> SNASSPSSPADWAKKLTDAVLRQKAGETLTAADRDFSNADFRNITFSKILPPSFMERDGDIIKGFNFSNSKFTYSDISHLHFDECRFTYSTLSDVVCSNTKFSNSDMNEVFLQYSITTQQQPSFIDTTLKNTLIRHKANLSGVILNEPDNSSPPSVSGGGNFIRLGDIWLQMPLLWTENAVDGFLNHEHNNGKSILMTIDSLPDKYSQEKVQAMEDLVKSLRGGRLTEACIRPVESSLVSVLAHPPYTQSALISEWLGPVQERFFAHQCQTYNDVPLPAPDTYYQQRILPVLLDSFDRNSAAMTTHSGLFNQVILHCMTGVDCTDGTRQKAAALYEQY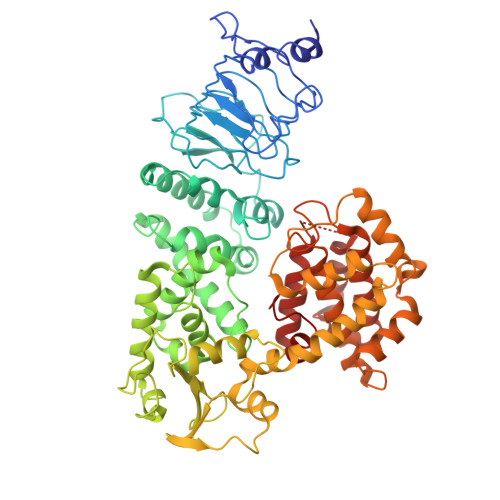LAHPAVSPHIHNGLFGNYDGSPDWTTRAADNFLLLSSQDSDTAMMLSTDTLLTMLNPTPDTAWDNFYLLRAGENVSTAQISPVELFRHDFPVFLAAFNQQATQRRFGELIDIILSTEEHGELNQQFLAATNQKHSTVKLIDDASVSRLATIFDPLLPEGKLSPAHYQHILSAYHLTDATPQKQAETLFCLSTAFARYSSSAIFGTEHDSPPALRGYAEALMQKAWELSPAIFPSSEQFTEWSDRFHGLHGAFTCTSVVADSMQRHARKYFPSVLSSILPLAWA> KLSLQDVAELIRARACQRVVVMVGAGI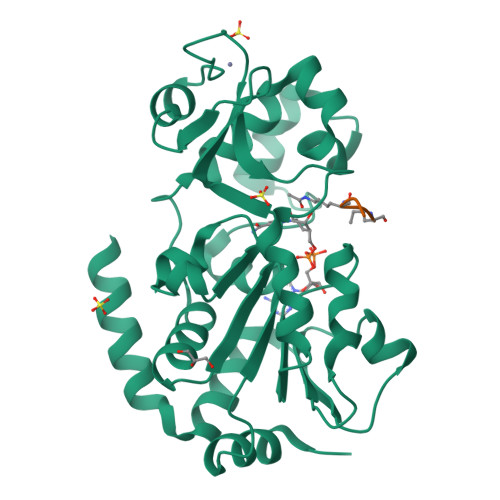STPSGIPDFRSPGSGLYSNLQQYDLPYPEAIFELPFFFHNPKPFFTLAKELYPGNYKPNVTHYFLRLLHDKGLLLRLYTQNIDGLERVSGIPASKLVEAHGTFASATCTVCQRPFPGEDIRADVMADRVPRCPVCTGVVKPDIVFFGEPLPQRFLLHVVDFPMADLLLILGTSLEVEPFASLTEAVRSSVPRLLINRDLVGPLAWHPRSRDVAQLGDVVHGVESLVELLGWTEEMRDLVQRETGKLD;> SGKVL Human gut commensal Bacteroidetes rely on multiple transport systems to acquire vitamin B12 and related cobamides for fitness in the gut. Here, we report the function and structural characterization of one of these proteins, BtuH, which binds vitamin B12 directly via a C-terminal globular domain that has no known structural homologs. This protein is required for efficient B12 transport and competitive fitness in the gut, demonstrating that members of the heterogeneous suite of accessory proteins encoded in Bacteroides cobamide transport system loci can play key roles in vitamin acquisition. Our data indicate that BtuH2 is a membrane-associated lipoprotein that binds vitamin B12 directly, suggesting a role for BtuH2 in cobamide capture at the cell surface.

The truncated protein includes residues 103 to 593 with a C-terminal His6 tag. This shorter version produced well-diffracting crystals, allowing us to solve the structure of cyanocobalamin-bound BtuH2(103-593)-His6 via cobalt-based single-wavelength anomalous diffraction (Co-SAD). The solved structure has three domains; two Ig-like N-terminal PKD domains (Ig-like 2 and 3 in the full-length protein) and a globular C-terminal domain. The N-terminal region shows high flexibility and is only well-structured in one of the two chains present in the asymmetric unit (chain A). As expected from the successful structure solution via Co-SAD, clear electron density is visible for a vitamin B12 molecule bound in a cleft on the C-terminal domain, allowing unambiguous placement of the ligand. There are two main regions of interaction between B12 and BtuH2: the tetrapyrrole ring and the nucleotide loop. Residues Tyr510, Trp577, Trp511, and His476 form hydrogen bonds with the amide functional group of the substituents in C-7, C-8, and C-13 of the tetrapyrrole ring, whereas Asn399 and Gln333 mediate polar interactions with the phosphate and the -CH2OH functional group of the ribose, respectively. The interaction between the dimethylbenzimidazole (DMB) lower ligand and BtuH2 is likely weak, consisting only of van der Waals interactions with Leu578 and Phe401. The nucleotide loop interactions, including those mediated by Asn399 and Gln333, and the lack of strong interactions with the lower ligand, suggest that BtuH2 primarily interacts with vitamin B12 via its tetrapyrrole ring and nucleotide loop, which are conserved across cobamides. After inspection of the residues surrounding the electron density, in silico analyses of the geometry and coordination using METALizer and the CheckMyMetal server, and the analysis of anomalous signal peaks we modeled these as one sodium and two calcium atoms. The calcium ion located at the interface between the Ig-like domain 3 and the B12 binding domain is coordinated only with amino acids from the globular domain.

>[2x]MGAEEELKVEVKELTPPVISLALPSQGLKVVRNTDYTFTPDIQHSDVEGFKIEWVREGKIVSTENTYTFNEKELGVYTVTINASNIDGTTTKDVSVEVVETMPYVVKFPTPSYLQTSTDRYTFADRPVFLRPLLEYFDNPRFEWSVDGQVMEGEVERMFKFTPSAPGEYTVSCTVSEDTPTEKISRNIDKGKTAVTATVKVVCVDKKEQDGFRASGSSKLWNKVYEYTPAPGQFINETSTIGGMTGNETSPEAAVAWATQRLKDKLHVSLGSFGGYIIVGFDHSIPNSGNQYDFCVQGNAFDGSSEPGIVWVMQDINGNGLPDDEWYELKGSEAGKEETIQNFEVTYYRPEGKKMDVQWISSDGRNGWVDYLSAYHTQDYYYPAWISENSYTLTGTCLAARNTQDSQTGYWDNQSYDWGYVDNFGNDQIEGGSTVDGSGQRNGFKISNAIHADGTEANLQYIDFIKIQCGVLAKSGWLGEVSTEVFSFEDLTKLEHHHHHH[(2S)-2-[(E)-octadec-10-enoyl]oxy-3-oxidanyl-propyl] 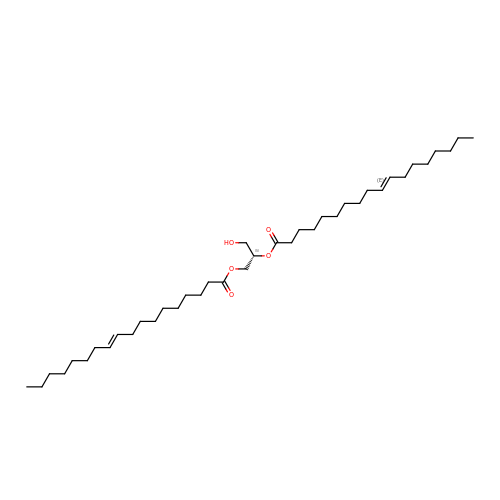octadec-10-enoate | C39 H72 O5 | UGRFXJLWUONJDY-NVXOQYPQSA-N>QTVTEPVGSYARAERPQDFEGFVWRLDNDGKEALPRNFRTSADALRAPEKKFHLDAAYVPSREGMDALHISGSSAFTPAQLKNVAAKLREKTAGPIYDVDLRQESHGYLDGIPVSWYGERDWANLGKSQHEALADERHRLHAALHKTVYIAPLGKHKLPEGGEVRRVQKVQTEQEVAEAAGMRYFRIAATDHVWPTPENIDRFLAFYRTLPQDAWLHFHAEAGVGRTTAFMVMTDMLKNPSVSLKDILYRQHEIGGFYYGEFPIKTKDKDSWKTKYYREKIVMIEQFYRYVQENRADGYQTPWSVWLKSHPA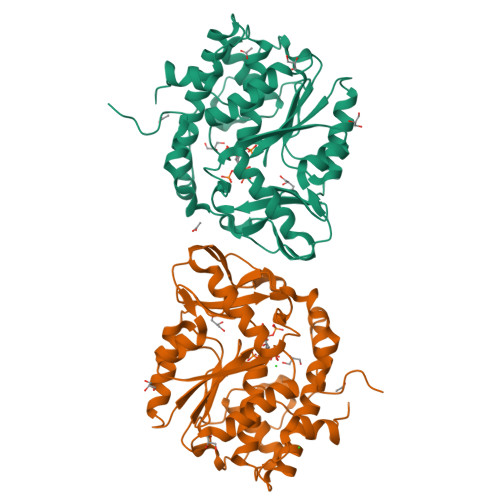KA[2x]2-(methylsulfanyl)adenosine 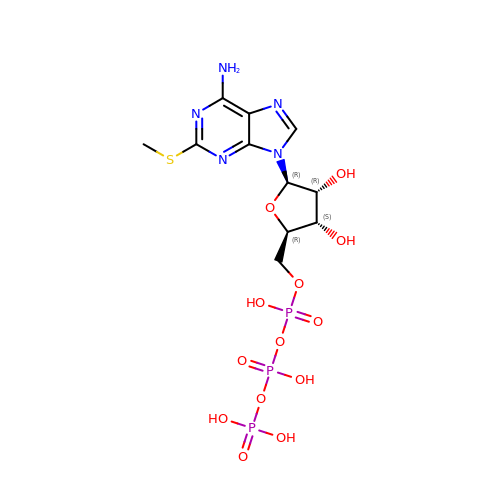5'-(tetrahydrogen triphosphate) | C11 H18 N5 O13 P3 S | XNOBOKJVOTYSJV-KQYNXXCUSA-N> LPQMTQQLNSDDMQEQLSATVKFRQILSREHRPPIDVVIQAG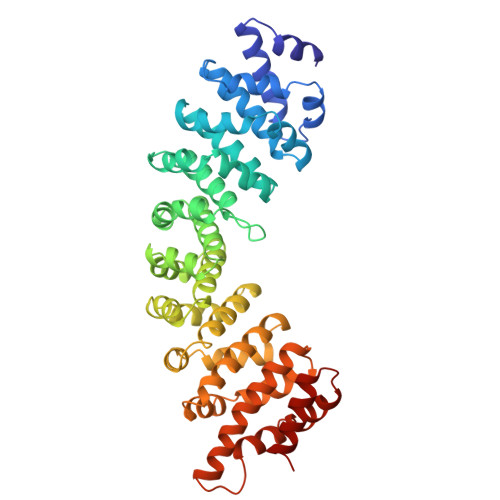VVPRLVEFMRENQPEMLQLEAAWALTNIASGTSAQTKVVVDADAVPLFIQLLYTGSVEVKEQAIWALGNVAGDSTDYRDYVLQCNAMEPILGLFNSNKPSLIRTATWTLSNLCRGKKPQPDWSVVSQALPTLAKLIYSMDTETLVDACWAISYLSDGPQEAIQAVIDVRIPKRLVELLSHESTLVQTPALRAVGNIVTGNDLQTQVVINAGVLPALRLLLSSPKENIKKEACWTISNITAGNTEQIQAVIDANLIPPLVKLLEVAEYKTKKEACWAISNASSGGLQRPDIIRYLVSQGCIKPLCDLLEIADNRIIEVTLDALENIIKMGEADKEARGLNINENADFIEKAGGMEKIFNCQQNENDKIYEKAYKIIETYFG>MKDMPAMPADTPSALLALAGEALPELESLQSRATEALRALVAPAGKPQPALLEQHQHAAHALSWLTTYVESIRQLSGWAGRLAEAGNLGRIEALILQIGLGEYLGQIAGGIPMSQTEFARLSDLELDWQPGEAAAKLMRGNTAPARAELARLMQDNHGRATFGATGLDEDLEMIRDQFRRYAEERVIPNAHEWHLKDQLIPMEIIEELAELGVFGLTIPEEFGGLGLSKASMVVVTEELSRGYIGVGSLGTRSEIAAELILCGGTEAQKAKWLPGLASGEILSTAVFTEPNTGSDLGSLRTRAVRDGEDWVVTGNKTWITHAQRTHVMTLLARTDPETTDWRGLSMFLAEKEPGTDDDPFPTPGMTGGEIEVLGYRGMKEYELGFDGFRIKGENLLGGEPGRGFKQLMETFESARIQTAARAVGVAQSAAEIGMRYAVDRKQFGKSLIEFPRVADKLAMMAVEIMIARQLTYFSAWEKDHGRRCDLEAGMAKLLGARVAWAAADNALQIHGG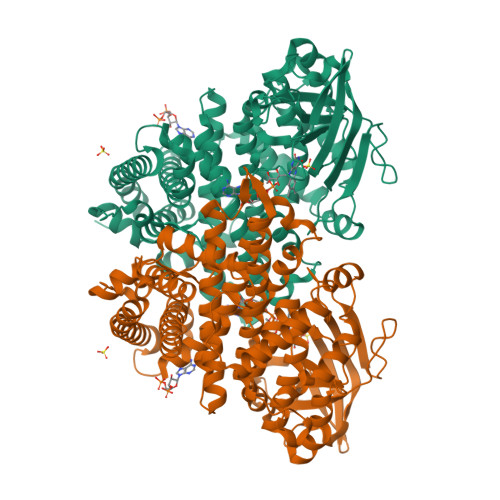NGFALEYAISRVLCDARILNIFEGAAEIQAQVIARRLLD[2x]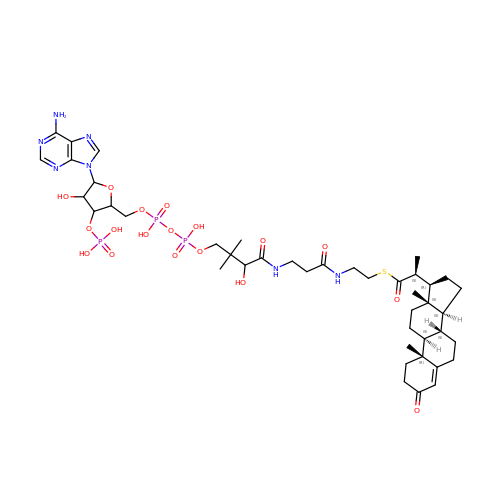3-oxo-23,24-bisnorchol-4-en-22-oyl-CoA | C43 H66 N7 O18 P3 S | CJJBDUCNUMWUJX-OFYMOSBZSA-N> IQTTAPPVKESSFVEKMKKTGRNIIVFYGSQTGTAEEFANRLSKDAHRYGMRGMSADPEEYDLADLSSLPEIDKSLVVFAMATYGEGDPTCNAQDFYDWLQETDVDLTGVKFAVFGLGNKTYEHFNAMGKYVDQRLEQLGAQRIFELGLGDDDGNLEEDFITWREQFWPAVAEFFGVEATGEESSIRQYELVVHEDMDVAKVYTGEMGRLKSYENQKPPFDAKNPFLAAVTANRKLNQGTERHLMHLELDISDSKIRYESGDHVAV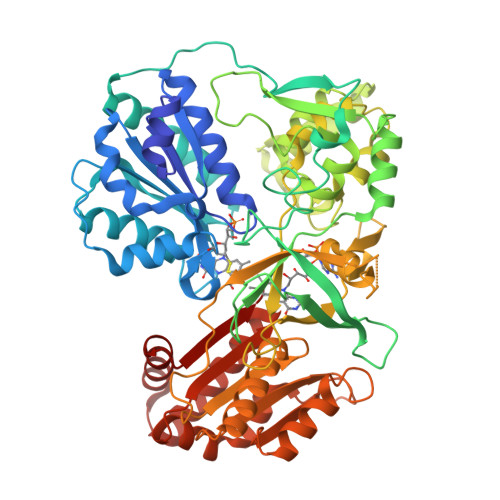YPANDSALVNQIGEILGADLDVIMSLNNLDEESNKKHPFPTPTTYRTALTYYLDITNPPRTNVLYELAQYASEPSEQEHLHKMASSSGEGKELYLSWVVEARRHILAILQDYPSLRPPIDHLLELLPRLQARYYSIASSSKVHPNSVHITAVAVEYEAKSGRVNKGVATSWLRAKEPAGENGGRALVPMFVCKSQFRLPFKSTTPVIMVGPGTGIAPFMGFIQERAWLREQGKEVGETLLYYGARRSDEDYLYREELARFHKDGALTQLNVAFSREQAHKVYVQHLLKRDREHLWKLIHEGGAHIYVCGDARNMAKDVQNTFYDIVAEFGPMEHTQAVDYVKKLMTKGRYSLDVWS>[2x]CGTGAAT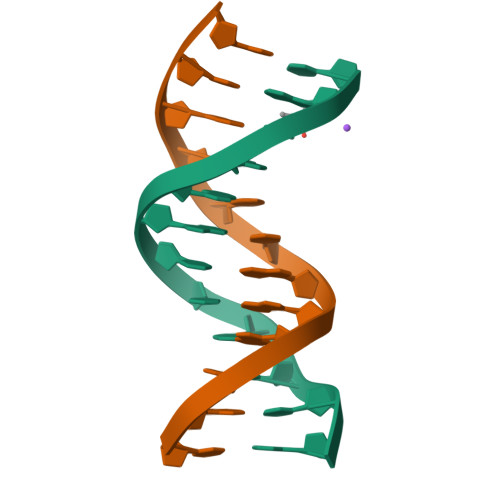TCACG>MHHHHMITLENPDIKYPLRLIDKEILSHDTRRFRFALPSPQHILGLPIGQHIYLSTRIDGNLV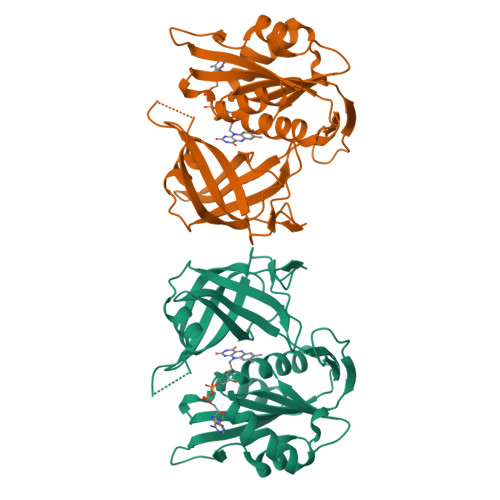IRPYTPVSSDDDKGFVDLVVKVYFKETHPKFPAGGKMPQYLENMNIGDTIEFRGPNGLLVYQGKGKFAIRADKKSNPVVRTVKSVGMIAGGTGITPMLQVIRAVLKDPNDHTVCYLLFANQSEKDILLRPELEELRNEHSSRFKLWYTVDKAPDAWDYSQGFVNEEMIRDHLPPPGEETLILMCGPPPMIQFACLPNLERVGHPKERCFTF[2x]>MRYQKVAIGIAQRIVDGKFPLGQKIKSRSTLASYFNVSPETARKAINVLADLDIVSVRQGSGVIVISRDKAIEYLEKFEATAGLKEMKQDIQRSLLKQKQELDAMNKMMDTFLSQASLIRKKFPFEPFELLLDHDSANLNKSLADLNLWHQTGATV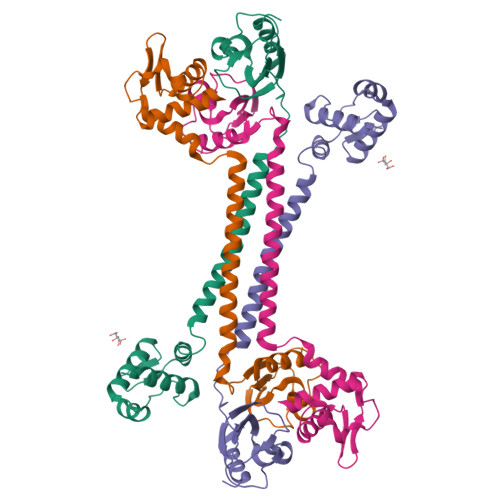VALKSKGELLLSPGPYATVRKGDILYFVGDDFAFSRMKNLFDLEHHHHHH[2x]> GSSKLLETIDQLHLEFAKRAAPFNNWMEGAMEDLQDMFIVHSIEEIQSLITAHEQFKATLPEADGERQSIMAIQNEVEKVIQSYNIRISSSNPYSTVTMDELRTKWDKVKQLVPIRDQSLQEELARQHANERLRRQFAAQANAIGPWIQNKMEEIARSSIQITGALEDQMNQLKQYEHNIINYKNNIDKLEGDHQLIQEALVFDNKHTNYTMEHIRVGWELLLTTIARTINEVETQILTRDAKGITQEQMNEFRAS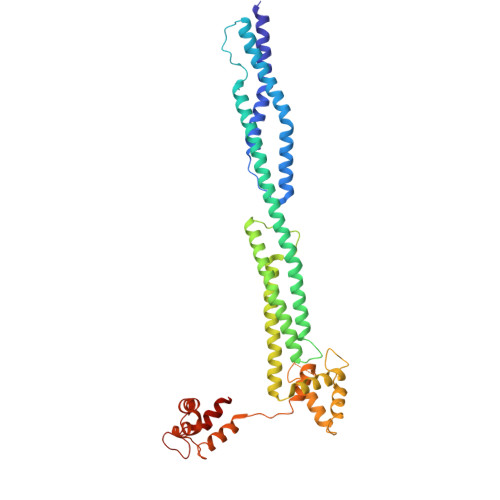FNHFDRRKNGLMDHEDFRACLISMGYDLGEAEFARIMTLVDPNGQGTVTFQSFIDFMTRETADTDTAEQVIASFRILASDKPYILAEELRRELPPDQAQYCIKRMPAYSGPGSVPGALDYAAFSSALYGESDL> GPMPGKKFVARVAEARAEDVGKRVVIIPKAE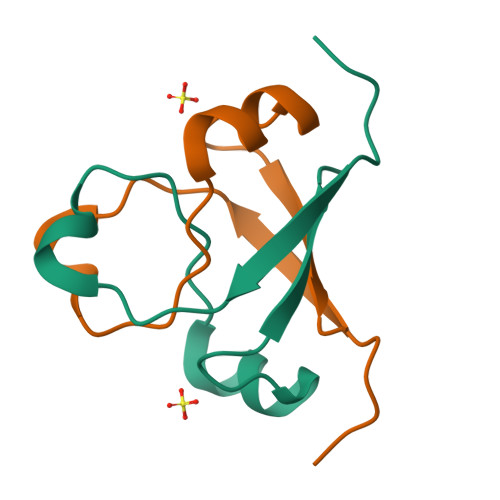RAKVGIKVGDVVEVKKV> REFAPPPNLPDPKFESKAALLAARGPEELLCFTERLEDLVCFWEEAASAGVGPGQYSFSYQLEDEPWKLCRLHQAPTARGAVRFWCSLPTADTSSFVPLELRVTAASGAPRYHRVIHINEVVLLDAPVG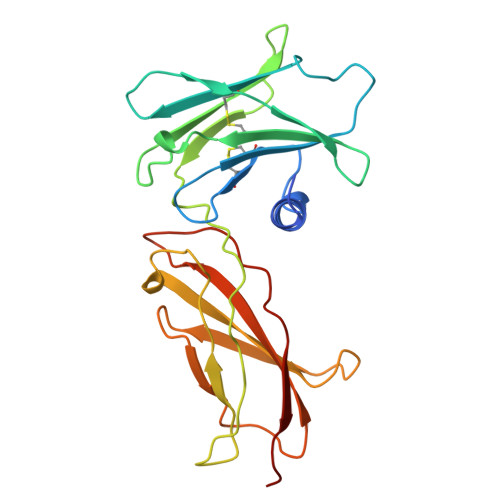LVARLADESGHVVLRWLPPPETPMTSHIRYEVDVSAGQGAGSVQRVEILEGRTECVLSNLRGRTRYTFAVRARMAEPSFGGFWSEWSEPVSLLTPSDLD> ATAVTGGGASLPADLYKGSADSILPANFSYAVTGSGTGKKAFLENNSALFSTTGTVHFAGSDSVLSSTELNTYNSTYNVSGDANRYGALVQIPSVATSVTIPFNKAGSAVDLSVTQVCGIFSGKITSWSQLAGLGRTGD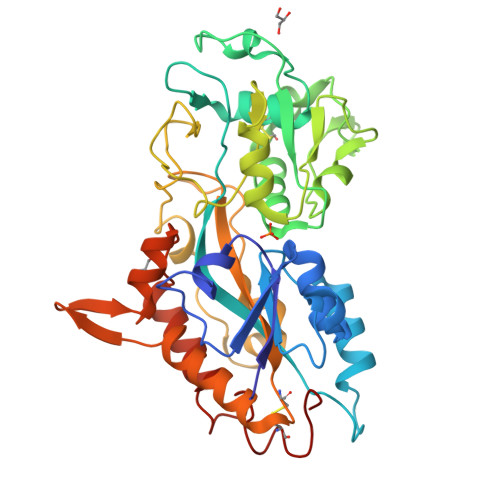IQVVYRGESSGTSELLTRFLTSACQPADVSSSNLKLTNGVPAFSVQSTFANLFTTVPSNFIAAPATGGTALYNAVYAIDGRVGYVGPDAIPSLTDATKVAKVKGFSPDEVSVQATLETAAPPTGAAAENPANWVPVFGNPSAGYPIAGYTNFVFGQCYKNATVGANVRGFLTKHYGSTVVNGVEQGPNDVAIRAHKFIPLTKAWRDAVRARFATATNAGAVNNPATCSGIGRPL>DPAGLLDLRQGMFAQLVAQNVLLIDGPLSWYSDPGLAGVSLTGGLSYKEDTKELVVAKAGVYYVFFQLELRRVVAGEGSGSVSLALHLQPLRSAAGAAALALTVDLPPASSEARNSAFGFQGRLLHLSAGQRLGVHLHTEARARHAWQLTQGATVLGLFRVTPEI[3x];>SLQDPCSNC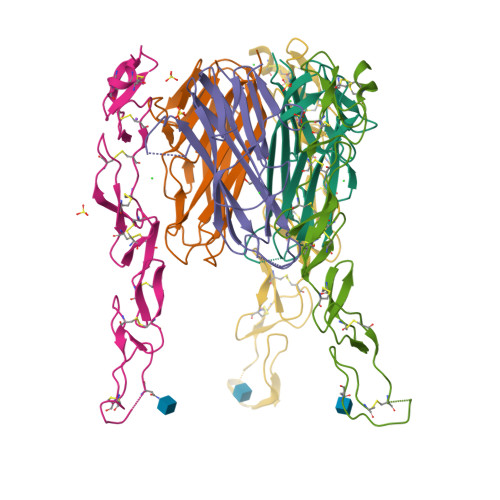PAGTFCDNNRNQICSPCPPNSFSSAGGQRTCDICRQCKGVFRTRKECSSTSNAECDCTPGFHCLGAGCSMCEQDCKQGQELTKKGCKDCCFGTFNDQKRGICRPWTNCSLDGKSVLVNGTKERDVVCGP[3x]> MERPQLDSMSQDLSEALKEATKEVHIRAENSEFMRNFQKGQVSREGFKLVMASLYHIYTALEEEIERNKQNPVYAPLYFPEELHRRAALEQDMAFWYGPHWQEAIPYTPATQHYVKRLHEVGGTHPELLVAHAYTRYLGDLSGGQVLKKIAQKAMALPSSGEGLAFFTFPSIDNPTKFKQLYRARMNTLEMTPEVKHRVTEEAKTAFLLNIELFEELQALLTEEHKDQSPSQTEFLRQR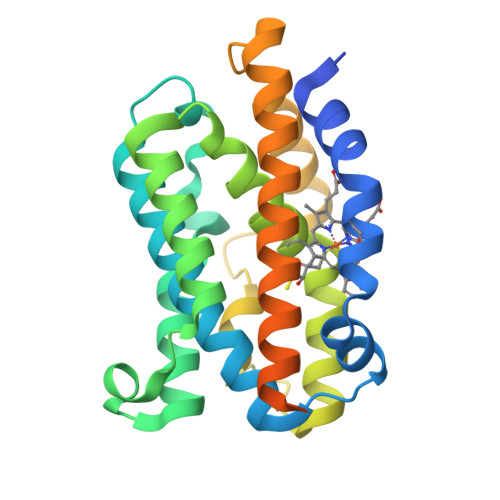PASLVQDTTSAETPRGKSQISTRL> QIHDITGKDCQDIANKGAKQSGLYFIKPLKANQQFLVYCEIDGSGNGWTVFQKRLDGSVDFKKNWIQYKEGFGHLSPTGTTEFWLGNEKIHLISTQSAIPYALRVELEDWNGRTSTADYAMFKVGPEADKYRLTYAYFAGGDAGDAFDGFDFGDDPSDKFFTSHNGMQFSTWD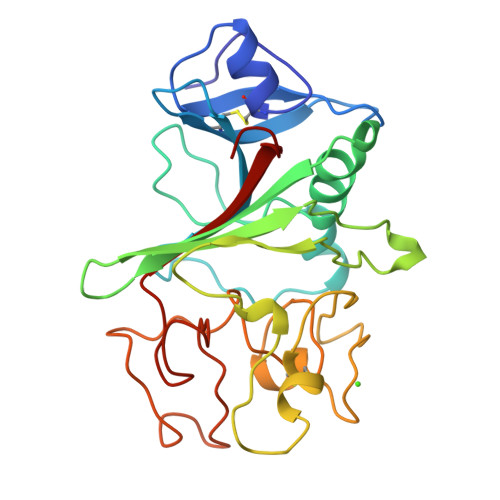NDNDKFEGNCAEQDGSGWWMNKCHAGHLNGVYYQGGTYSKASTPNGYDNGIIWATWKTRWYSMKKTTMKIIPFNRL Lysophosphatidic acid receptor 1 (LPA1) is one of the six G protein-coupled receptors activated by the bioactive lipid, lysophosphatidic acid (LPA). LPA1 couples to the G proteins such as Gαi, Gαq, and Gα12/13, and transduces various intracellular signals, e.g., increased Ca2+ concentration and actin reorganization by the Rho/ROCK pathway. LPA1 is widely expressed in several organs to control cell proliferation and survival, cell–cell contact, cell migration, and cytoskeletal morphological changes. LPA1 is associated with various diseases such as cancer, inflammation, and neuropathic pain, and thus is a pathologically important receptor that is an essential drug target.

ONO-0740556 provides an extensive interaction network with N-term, ECL1, 2, and TMs 2, 3, 5, 6, and 7 of the receptor. The binding site consists of a polar recognition region on the extracellular side and a hydrophobic pocket within the transmembrane region. The head phosphate and glycerol moieties of ONO-0740556 are located in the polar recognition site. Two oxygen atoms of the head phosphate form salt bridges with K39N-term and R1243.28 (superscripts indicate Ballesteros–Weinstein numbers). The phosphate group also forms a hydrogen bond with Y34N-term, and is tightly recognized by the positively charged resides K2947.36. Moreover, the nitrogen atom in the amide bond forms a hydrogen bond with E2937.35. By contrast, the long acyl chain fits into the transmembrane pocket in a bent conformation and forms extensive hydrophobic interactions with the receptor. Notably, the aromatic moiety in the middle of the acyl chain is sandwiched between two leucines, L2786.55 and L2977.39. Furthermore, in the acyl chain, the C14 carbon forms a CH–π interaction with W2105.43.

> DYKDDDDAMGAAISTSIPVISQPQFTAMNEPQCFYNESIAFFYNRSGKHLATEWNTVSKLVMGLGITVCIFIMLANLLVMVAIYVNRRFHFPIYYLMANLAAADFFAGLAYFYLMFNTGPNTRRLTVSTWLLRQGLIDTSLTASVANLLAIAIERHITVFRMQLHTRMSNRRVVVVIVVIWTMAIVMGAIPSVGWNCICDIENCSNMAPLYSDSYLVFWAIFNLVTFVVMVVLYAHIFGYVRQRTMRMSRHSSGPRRNRDTMMSLLKTVVIVLGAFIICWTPGLVLLLLDVCCPQCDVLAYEKFFLLLAEFNSAMNPIIYSYRDKEMSATFRQILCCQRSENPTGPTEGSDRSASSLNHTILAGVHSNDHSVVENLYFQ Here we report a structural and functional analysis for an epimerase, KasQ, that primes KSM biosynthesis rather than the previously proposed KasF/H, which instead acts as an acetyltransferase, inactivating KSM. Our biochemical and biophysical analysis determined that KasQ converts UDP-GlcNAc to UDP-ManNAc as the initial step in the biosynthetic pathway. To better understand the catalytic mechanism of KasQ, we solved crystal structures of KasQ for the wild type (WT) and its complexes with UDP or UDP-Glc in resolutions of 2.44 Å, 2.58 Å, and 2.09 Å, respectively. In brief, each monomer consists of two domains (N-terminal and C-terminal domains), in which each subdomain is made of a typical sandwich (αβα) architecture of a Rossmann fold.

Despite this, the structures, not least the one with UDP-Glc, are still in a position to provide a structural basis to help elucidate the mechanism of the epimerization reaction mediated by KasQ. In view of the KasQ–UDP-Glc complex, the UDP portion is well defined as it is surrounded by an array of highly conserved residues, His209, Leu267, Ser286, Gly287, and Gly289. The hexose moiety is held in place by a group of highly conserved residues for its recognition and epimerization, except for Arg12, which differs from the corresponding residues in other homologs pointing away from the uracil O2 atom (4.6 Å); the guanidino group of Arg309, which is associated with Glu291 (2.9 Å), is in close proximity to the C2 hydroxyl group (4.1 Å), and the terminal carboxyl group of Asp97 is in close proximity to the C2 atom (3.8 Å). These residues may act as a set of the interlinking acids/bases triggering the elimination/addition reaction for the epimerization of UDP-GlcNAc to UDP-ManNAc. The C3 hydroxyl group of the hexose moiety is also within hydrogen-bonding distances to both the guanidino group of Arg309 (2.7 Å/2.9 Å) and the carboxyl group of Glu119 (3.3 Å). The C4 hydroxyl group is interacting with both Lys17 and Gln95 through hydrogen bonding (3.5 Å and 3.1 Å, respectively). The C6 hydroxyl group is likewise interacting with the carboxyl and amino groups of Asp97 through hydrogen bonding (2.5 Å and 2.8 Å, respectively). Importantly, the carboxyl group of Asp97 that is located on top of the sugar plane relative to the C2 atom (3.8 Å) likely serves as the general base to deprotonate C2 in the first half of the reaction, yielding AAG and UDP; the Arg309/Glu291 dyad, on the other hand, acts as the general acid, likely protonating AAG to afford UDP-ManNAc, thus completing the epimerization reaction. Q95 was found interacting with the C4-OH of UDP-Glc in contrast to the histidine (H) counterpart in homologous 2-epimerases, which is at a distance from C4-OH of 4.5 Å. Despite the fact that KasQ exists as dimers in solution as well as asymmetric units, only one UDP-Glc molecule is bound to one protomer of the dimer.

>SHMALRVGIVYGTRPEAIKLAPLVLALDADPGFEPVIITTGQHRDMLDEINELFGLRPRHNLDIMRPGQRLSAMASRIVGELGDPLLDELVDVAVVQGDTSTAFAAAYAAACERIPVAHLEAGLRTGDRFEPFPEEINRRLITQLADLHFAPTADAAGNLLAEGVRSDDVYVTGNTVIDAMHLVLDRPGDSANRELDAFTEGRQTVLLTMHRRESWGIPMGRVAAAVAELCRSRPTLRFVIPLHPNPEVRRVFRSHLSSLTQVLLCEPLRYSEFIRLMHRAVLVLTDSGGVQEEAPTLGKPVLVLRDRTERPEGIAAGCARLVGTDPALIVKEVGRLLDDPEAYEAMRRPGIVCYGEGDAAARCLEALRERWLSSPDASAGLRTYR[8x]> MELRVGNRYRLGRKIGSGSFGDIYLGTDIAAGEEVAIKLECVKTKHPQLHIESKIYKMMQGGVGIPTIRWCGAEGDYNVMVMELLGPSLEDLFNFCSRKFSLKTVLLLADQMISRIEYIHSKNFIHRDVKPDNFLMGLGKKGNLVYIIDFGLAKKYRDARTHQHIPYRENKNLTGTARYASINTHLGIEQSRRDDLESLGYVLMYFNLGSLPWQGLKAATKRQKYERISEKKMSTPIEVLCKGYPSEFATYLNFCRSLRFDDKPDYSYLRQLFRNLFHRQGFSYDYVFDWNML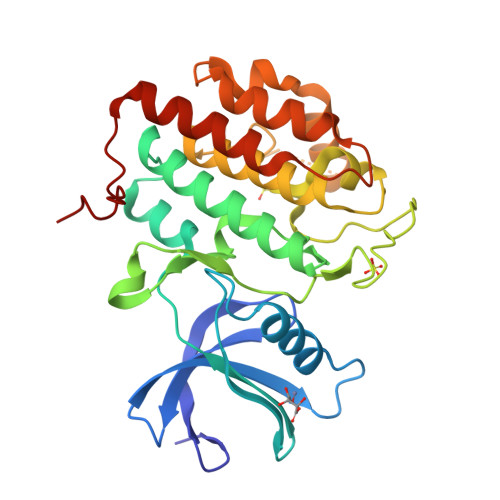K> AMGSPIFGYSNTQQSQRVVTADNLMYLRSGFAIDAIGTTVNNLVGGPVQGTNGGVLRAPIALDQLQSVEVTSGLYNWGGYHIVAIKFTMKDGSSVLLGSTHYASNK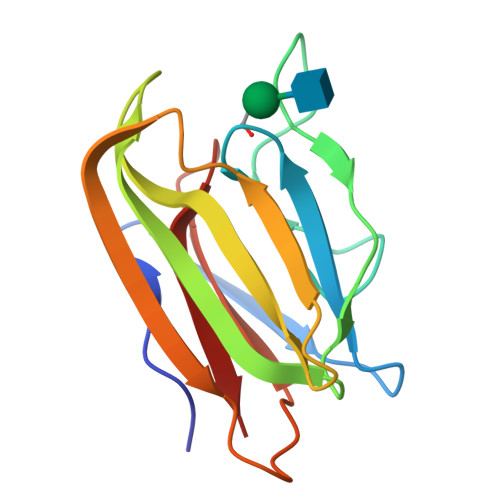KVETYTVPQGKRIKQINVWTGGWLVEGFQFVY> GDRVAGQVNSRRGELLELAAAMFAERGLRATTVRDIADGAGILSGSLYHHFASKEEMVDELL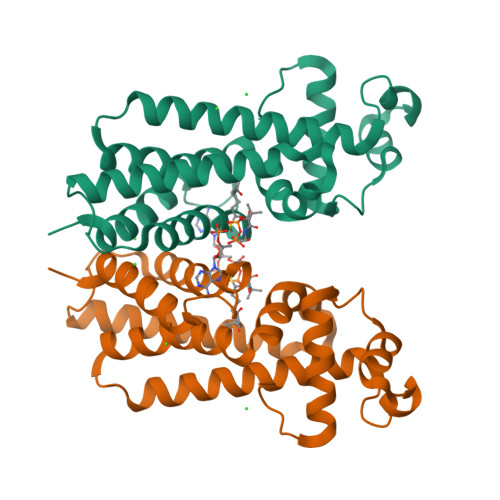RGFLDWLFARYRDIVDSTANPLERLQGLFMASFEAIEHHHAQVVIYQDEAQRLASQPRFSYIEDRNKQQRKMWVDVLNQGIEEGYFRPDLDVDLVYRFIRDTTWVSVRWYRPGGPLTAQQVGQQYLAIVLGGITKEGV(1S,2R,3S,4R)-4-(6-aminopurin-9-yl)cyclopentane-1,2,3-triol | C10 H13 N5 O3 | 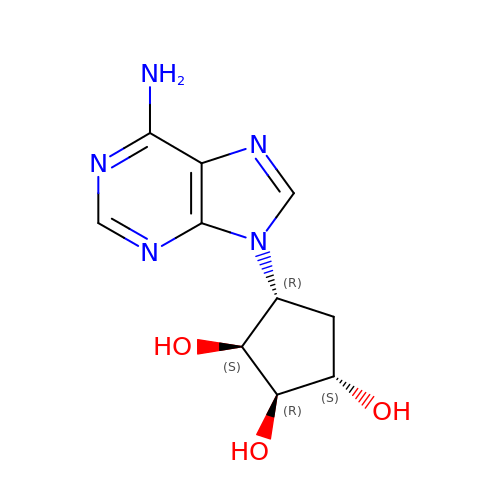VFKHECGAEJNAMV-HETMPLHPSA-N> MGSSHHHHHHSQDPMEIDELTALGGLLHDIGKPVQRAGLYSGDHSTQGARFLRDLAENTGRAEYELLSLFSEFHHKGHMKNDELMIRRIKELSPERFGLTMEDVLNALWIVYEADNLASGEREEGQPQASRPLYSVFNPGKAYPWAELDFEKELPVPGDVFSIRSQDYRELVKRLWEELSKAKLRSDRLLPVLEKYLTFVSSVTSEGNIISLYDHMRMTSAIALAMLRAGCTAEDVRSGRCRKEKRFLLIEGDFSGIQDFIYRVSGKGTLKYLRARSAYLELIGWDVVLEILSRLGLTRANVVFNAGGHFMIIAQNTPDAVKELEEIRAKAVEWLYREFESDLYLAIEWEPVSGREFGREGGKNLFAEARKRLKHKLTVRKLKRFGEIKGLFEHGHTERLAECPVCGRELPEGKLEPSASDPETKVCPTCNRLVSLGGNLPKLLGFGRTAKNDAGVLVEGPFSGFVPYLQGGRPVGEQILVKNTLNPGEIPESAQFVPYFVADYFKKDPKGGVATFEEL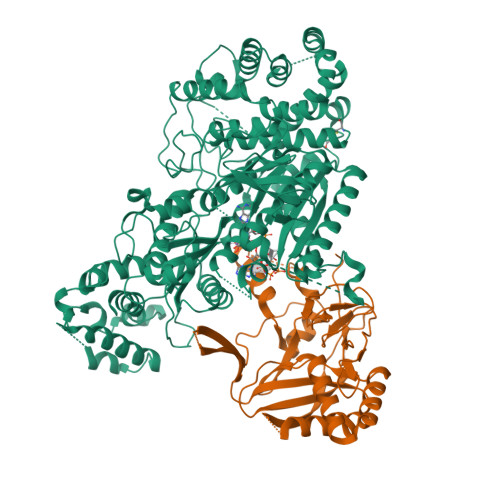SMASTGTRRLGVMKGDVDRLGEFFSSMDSPSKLATASRFMDYFFKGYIGAIIEGKFGYIIGDVPSLRDWPEEPDIVVVYAGGDAFFIVGAWDQIFELAFRVRRAFNAYTGGKLTLSVGLGYFDERTPIYRMADVVSERLDTAKDEGRNRVFVVGRSRPLDGKHKLSYEWNHYEELWRTYAPRIYAGNGRLKGKLESKKGLLWKLLEIRELYVRDPNDVRWAYLTAYLLGRHGLSDLFPELVGIDTKAVERKEPQPVYWVDGVLKIVLMAVRR;> MPKFIAVKLIPKGPFRDIPRADTLFGAIGNAISAIHGQSAVEELVDAFVGGARISSAFPYSGDTYYLPKPLSVEPALEGILTGLDEEERYTTAKRLRKAKYLDLKNFELALRLRPFTIPEEIPYARVDVPRVVLDRVTQDSSIYFWEEIRFREKSGVYFLYSGPREVFDGYIAPAMRFLGDTGIGGKSTWGAGLFEVEFHEMKIDAPGSEYSVTLSNALPTKTPVLWRLLRKGGWSFGRRKPRMTFIAEGSIVKNDPGGMERLELGLSHEVYVYGLTFPLGVELPEGLE> GAMGSDEQPHIGNYRLLKTLGKGNFAKVKRARHILTGREVAIKIIDKTQLNPTSLQKLFREVRIMKILNHPNIIKLFEVIETEKTLYLIMEYASKGEVYDYLVEHGRMKEKEARSKFRQIVSAVQYCHQKRIVHRDLKAENLLLDADMNIKIADFGFSNEFTKGGKLDTFCGSPPYAAPELFQGKKYDGPEVDVWSLGVILYTLVSGSLPFDGQNLKELRERVLR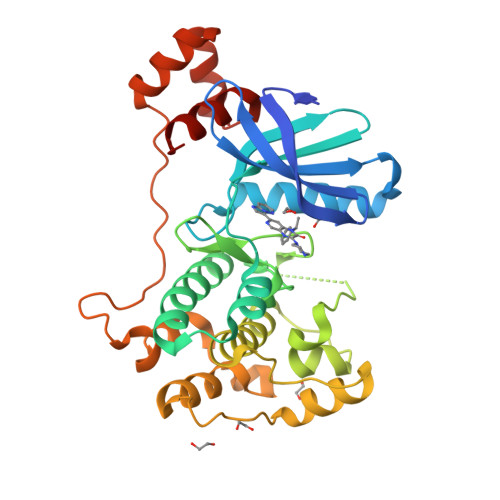GKYRIPFYMSTDCENLLKRFLVLNPIKRGTLEQIMKDRWINAGHEEDELKPFVEPELDISDQKRIDIMVGMGYSQEEIQESLSKMKYDEITATYLLLGRKSSE> MICIIMGSESDLKIAEKAVNILKEFGVEFEVRVASAHRTPELVEEIVKNSKADVFIAIAGLAAHLPGVVA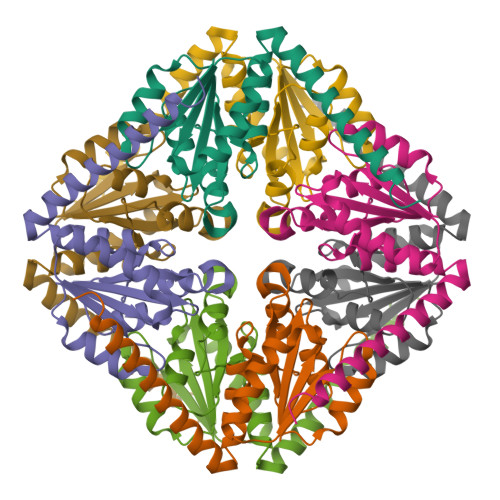SLTTKPVIAVPVDAKLDGLDALLSSVQMPPGIPVATVGIDRGENAAILALEILALKDENIAKKLIEYREKMKKKVYASDEKVKEMFK DITERCALINIUM | C46 H50 N6 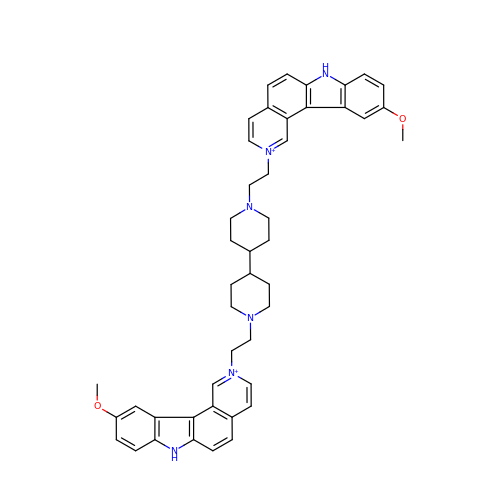O2 | NHUWXMNVGMRODJ-UHFFFAOYSA-P> MSIPNSFIIVGSGVFGLSLAYALSLDDRFADKKIILVDRWNFEPPNATGSVHNPAAANADTSRVIRRDYPHGPYASLALEAMKHWRGKFGENNRYVNQRLLFSGEGSSLTTPPKALETVNYIKKAYAISCELTPGGRDAVQVLDSLDEVRAFLGNTPSHPPHLPVNKDPAARDLRGYVSNDCGWADAGASIEWLRQEVLRLGRVECVVGEVESLVYSDDQRAVKGVKLVDGKVLTAELTVIAAGARSSHILGIPKLCDVYSEFVAYIQLTKEEADELRRRQWPILVNCHRGVFAVGPDHDNCLKFGHFSYSGIVDVLREASIQVPTRPDGWEAQQKYWSDPRFAFGGEVKVSALGDVDDYENPAAQRALADYRLFLLELLGPTGLQGVDTLGLDQSDNLLNNIANRPFTRVRKCWYNDTPALDFVVDYHPSYGKTLFVATGGCDHAFKFLPIIGEKTLALILRNRGDSAVSLPAGVEPSLEELSELWRFPVELLQDN

Recently, it was found that a biosynthetic gene cluster of Aspergillus fumigatus harbors a gene, termed fsqB (fumisoquin biosynthesis gene B) that encodes a flavoprotein belonging to the family of amine oxidases and catalyzes an oxidative cyclization yielding an isoquinoline ring system via C–C bond formation. Thus, the reaction reported for FsqB diverges from the canonical reaction scheme because the imine is not hydrolyzed but subject to nucleophilic attack by the catechol moiety of the substrate. Our study showed that FsqB structurally belongs to the amine oxidase family of flavoproteins and has an active site that is similar to well characterized enzymes of this family, notably MSOX, MTOX, and NikD. In summary, our study has shown that FsqB is a member of the family of amine oxidases, but in contrast to previously characterized members of this family, it combines the oxidation of a N-methyl group with the generation of a heterocyclic ring system.

We determined the crystal structure of FsqB to a resolution of 2.6 Å. The asymmetric unit of the hexagonal crystals contained only one protein chain, but an analysis using the EBI-Pisa server indicated the existence of a dimeric assembly involving a symmetry-related molecule generated by a crystallographic 2-fold symmetry axis. In this assembly, ∼2900 Å2 of solvent-accessible surface are buried on each protomer, predicting that this dimer should also be formed and stable in solution. The FsqB protomer consists of two discontinuous domains, an FAD-binding domain (residues 1–97, 183–257, and 419–496) and a substrate-binding domain (residues 98–182 and 259–418). The FAD-binding domain exhibits a three-layer ββα-fold with the diphosphate group of FAD bound at the C-terminal edge of a mostly parallel, central β-sheet. The most prominent feature of the substrate-binding domain is a seven-stranded, mostly antiparallel β-sheet, which spans across the bound flavin. The two N-terminal strands of this sheet wrap around the dimethyl-benzene part of the isoalloxazine ring system and provide the amino acid residue Cys-414, which is covalently bound to the 8α-methyl group of the FAD cofactor. The substrate-binding domain is also responsible for dimer formation. The central portion of the interface between the two protomers is formed by a long α-helix situated on top of the seven-stranded β-sheet as well as by surrounding loop regions. The active site of FsqB is located at the interface between the FAD binding and the substrate-binding domain at the core of the protein and is connected to the solvent by a long and rather broad tunnel.>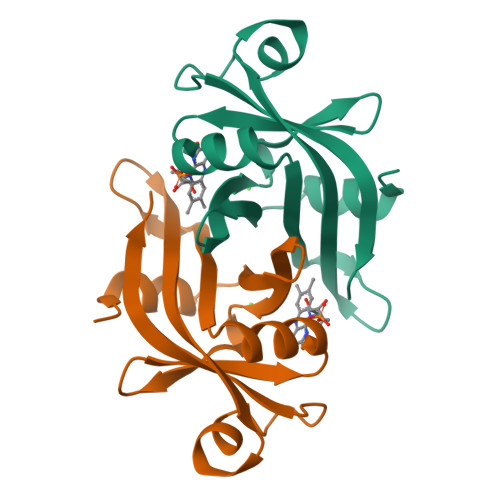[2x]MLPGTFFEVLKNTGVVAIATQGEDGPHLVNTWNSYLKVLDGNRIVVPVGGMHKTEANVARDERVLMTLGSRKVAGRNGPGTGFLIRGSAAFRTDGPEFEAIARFKWARAALVITVVSAEQTL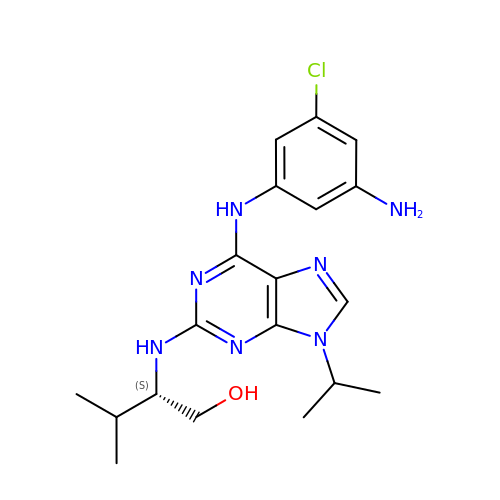(2S)-2-({6-[(3-AMINO-5-CHLOROPHENYL)AMINO]-9-ISOPROPYL-9H-PURIN-2-YL}AMINO)-3-METHYLBUTAN-1-OL | C19 H26 Cl N7 O | RAMROQQYRRQPDL-OAHLLOKOSA-N>MKAVLEQFGFPLTGTEARCYTNHALSYDQAKRVPRWVLEHISKSKIMGDADRKHCKFKPDPNIPPTFSAFNEDYVGSGWSRGAMAPAGNNKFSSKAMAETFYLSNIVPQDFDNNSGYWNRIEMYCRELTERFEDVWVVSGPLTLPQTRGDGKKIVSYQVIGEDNVAVPSHLYKVILARRSSVSTEPLALGAFVVPNEAIGFQPQLTEFQVSLQDLEKLSGLVFFPHLDRTSDIRNICSVDTCKLLDFQEFTLYLSTRKIEGARSVLRLEKIMENLKNAEIEPDDYFMSRYEKKLEELKAKEQSGTQIRKPSHHHHHH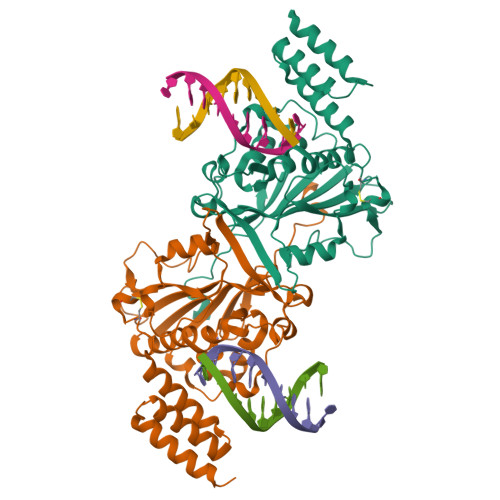[2x]> MEFSPPLQRATLIQRYKRFLADVITPDGRELTLHCPNTGAMTGCATPGDTVWYSTSDNTKRKYPHTWELTQSQSGAFICVNTLWANRLTKEAILNESISELSGYSSLKSEVKYGAERSRIDFMLQADSRPDCYIEVKSVTLAENEQGYFPDAVTERGQKHLRELMSVAAEGQRAVIFFAVLHSAITRFSPARHIDEKYAQLLSEAQQRGVEILAYKAEISAEGMAL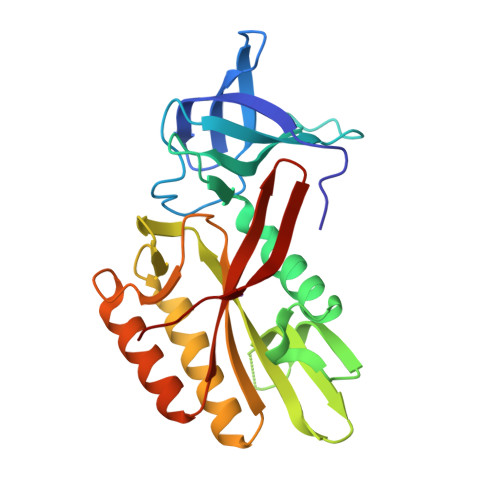KKSLPVTL> GYDKDLCEWSMTADQTEVETQIEADIMNIVKRDRPEMK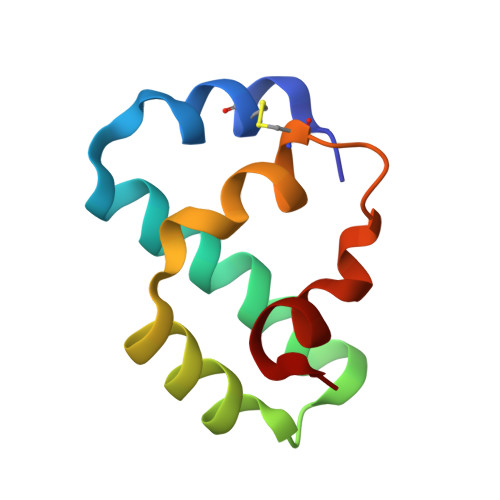AEVQKQLKSGGVMQYNYVLYCDKNFNNKNIIAEVVGE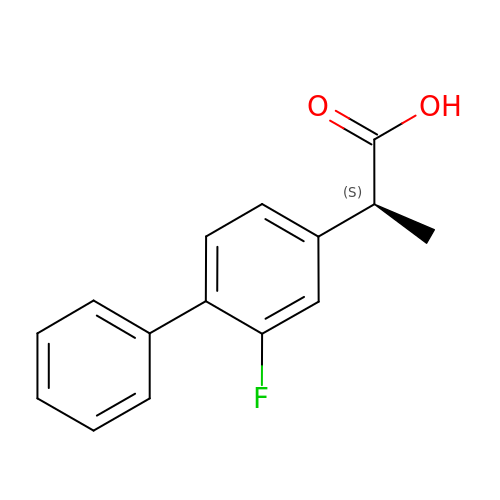FLURBIPROFEN | C15 H13 F O2 | SYTBZMRGLBWNTM-JTQLQIEISA-N> SSGHMKLTLENFYS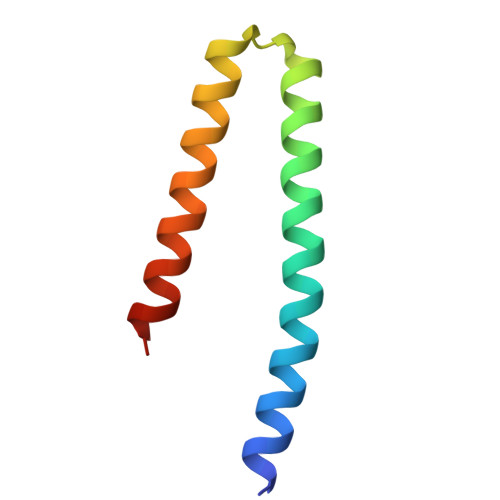NLILQHEERETRQKKLEVAMEEEGLADEEKKLRRSQHARKETEFLRLKRTRLGL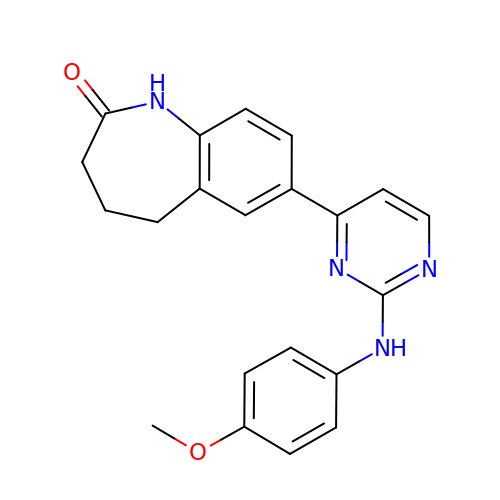7-[2-[(4-methoxyphenyl)amino]pyrimidin-4-yl]-1,3,4,5-tetrahydro-1-benzazepin-2-one | C21 H20 N4 O2 | RJPKXYNMTYJNMH-UHFFFAOYSA-N(~{Z})-7-[(1~{R},5~{S})-2-oxidanylidene-5-[(~{E},3~{S})-3-oxidanyloct-1-enyl]cyclopent-3-en-1-yl]hept-5-enoic 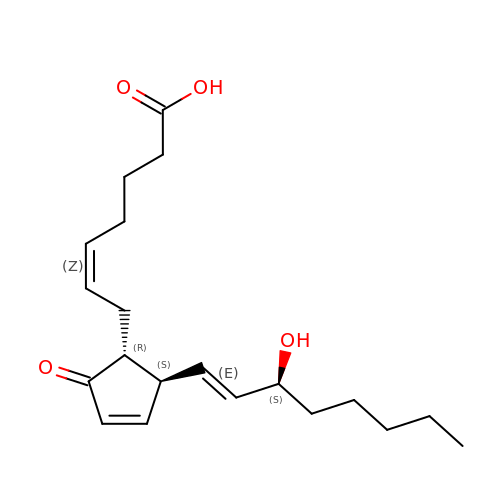acid | C20 H30 O4 | MYHXHCUNDDAEOZ-FOSBLDSVSA-N> MITNPGPLRVAYSPDYLDWLYRAYRSKLKYTDERKKAEEVFNGLLLTNQTDEQGPAAGAALPGAPPPGQTLRPRHSVRRQAGEARRAAAQAKLDTLAKQQGMLDLFERQPQFPAIHIDKAARFHVVELFKEMVLDRAWK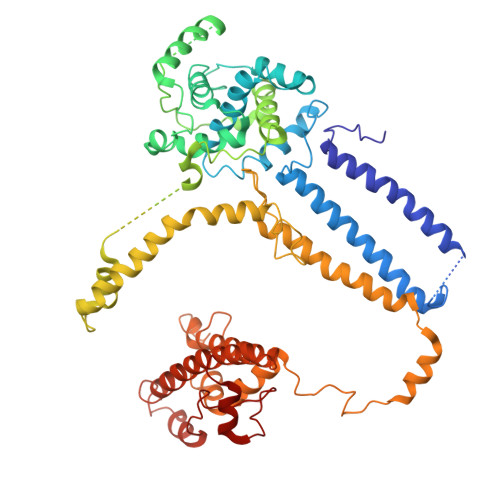PEEVWDKALLYRAILTERQASYPASYRYILDTAQRVNLAPRESGSSDTGSSSSSADARSSNESAGGIVSESTLVIPREDNYMYFVYLVRRYYIDNAVEGHVVLRCHRQPNASELLFSHPPPKDEHEVLRSLYRPGTATATQGKDASAKAQDGAATAPQQRPSGAATIARPRPPSSYPPIEALWRCEENEALLRVLVFGELNLLVSENPFVRFPKAQAYLTRPSASTPVPGAAGGSVEGADGYGGPQQQRRGGGHRGIGSDGGISLSSVIAEKRGHLLAPLSRNVAMMIDSRANDVRRLQQRYEREDTASFQKMLRGSAQVEENPGLYSAYSDWSYFNPRAVRAEERDALSRQTVAALKTYDEASRDIYRVGFEEAEARSAVRPVEGVNNAPSYVPTLPHFVALVKKDPHVSFLSHVALPEVYNTASHAAAGVSAKHQLEKLVVQLARALYRTALEFHKEQLRRVNRQKVQVAASLLDRFVTERWRVHCVAHPSSEGVRDMARRFRAYVPFEGRILDESGFPTDARVEDYERWMAAPSV>[2x]MGSSHHHHHHSSGLVPRGSHMASGLYPSYNTSP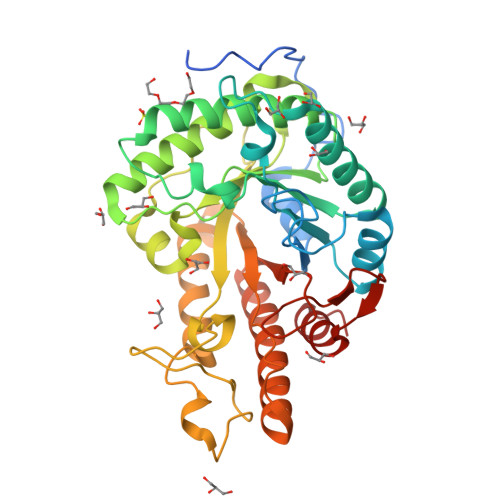AAPDSTGMQSTAVQLAGKIRLGWNIGNTMEAIGGETAWGNPMVSNELLKLVKDSGFDAVRIPVAWDQYANQESAEISAAWLNRVKQVVQMAIDNELYVLINIHWDGGWLENNITPAKKDENNAKQKAFWEQIATHLRDFDEHLLFAGTNEPNAENAEQMDVLNSYLQTFVDAVRSTGGKNAYRVLVLQGPVTDIEKTNELWTHMPADTATDRLMAEVHFYTPYNFALMRQDESWGKQFYYWGEGFLSTTDTERNPTWGEEATIDQLFDLMKTKFVDQGIPVVLGEFSAMRRTNLTGDALTLHLAGRAYYHKYVTQQALARGLLPFYWDNGGNDNFSSGIFNRQQNTVFDQQVLDALLEGAGAQ>MEVCLPNGHQVVDLINNAFEGRVSIYSAQEGWDKTISAQPDMMVCGGAVVCMHCLGVVGSLQRKLKHLPHHRCNQQIRHQDYVDVQFADRVTAHWKRGMLSFVAQMHEMMNDVSPDDLDRVRTEGGSLVELNWLQVDPNSMFRSIHSSWTDPLQVVDDLDTKLDQYWTALNLMIDSSDLIPNFMMRDPSHAFNGVKLGGDARQTQFSRTFDSRSSLEWGVMVYDYSELEHDPSKGRAYRKELVTPARDFGHFGLSHYSRATTPILGKMPAVF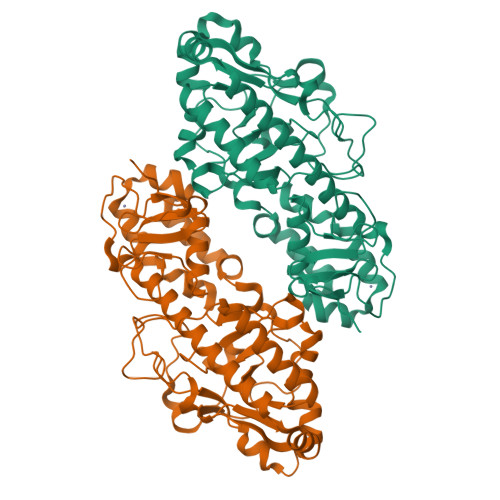SGMLTGNCKMYPFIKGTAKLKTVRKLVEAVNHAWGVEKIRYALGPGGMTGWYNRTMQQAPIVLTPAALTMFPDTIKFGDLNYPVMIGDPMILG[2x]> GAASNKSTSSAMSGSHQDLSVIQPIVKDCKEADLSLYN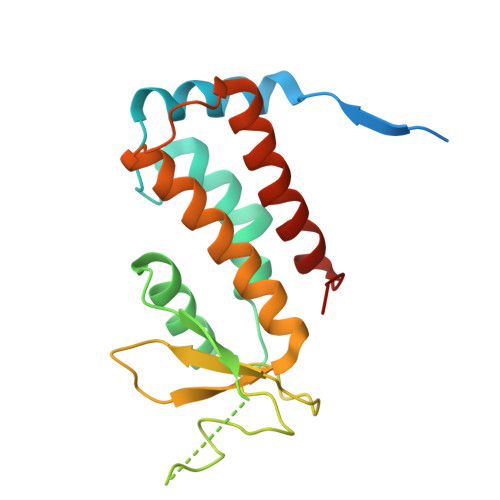EFRLWKDEPTMDRTCPFLDKIYQEDIFPCLTFSKSELASAVLEAVENNTLSIEPVGLQPIRFVKASAVECGGPKKCALTGQSKSCKHRIKLGDSSNYYYISPFCRYRITSVCNFFTYIRYIQQGLVKQQDVDQMFWEVMQLRKEMSLAKLGYFKEEL>NGGVGVDVELITSINVENDTFIERNFTPQEIEYCSAQPSVQSSFAGTWSAKEAVFKSLGVKSLGGGAALKDIEIVRVNKNAPAVELHGNAKK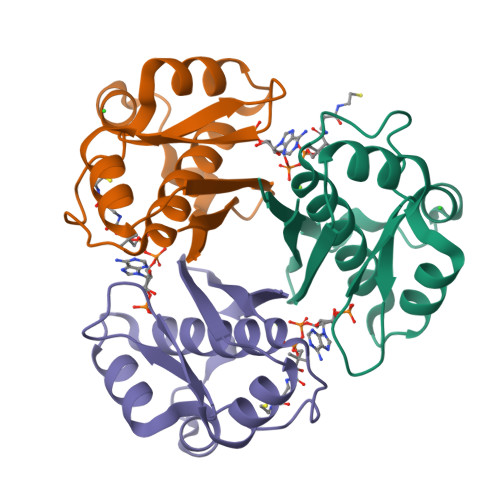AAEEAGVTDVKVSISHDDLQAVAVAVSTKK[6x]>MNAIGNFLVGTPVFTIFICLALGYLLGKLKIGSFTLGATVGVLIVALLIGQLGVFPRDTLLGDIFFDFFMFAIGYR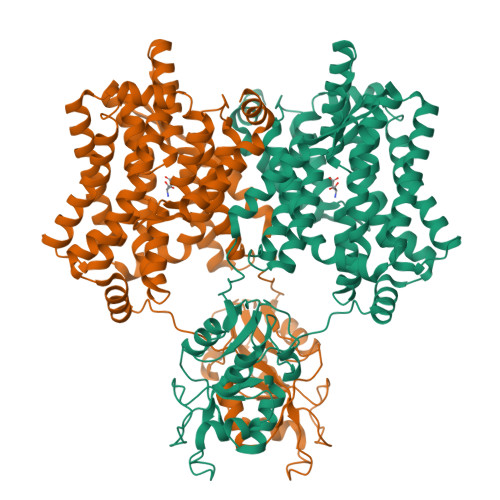VGPSFISSMKKFGAKIVYATLIFLVSAFIVAYACFKMFHIGPGIAAGIIAGGLTQSAVIGSSLETISKLPISDHLKTLYSNQIPIVYTLTYVFGTIGVLIFLRDIMPKLMHIDLKKQAVKTAKELDMIPVPVIVASTHFYTINDGSSLIGQTLGTVNTKFAKGLVAAGLNDSADMASVINAGDVLAISGGIDEIGRAVQEFNLLEVTGKTKAYVSKQVVLKKNFSADVLKNAQDKGVLVATLAGDVMDPAQFSTLKPAESVTLVGQKDAVSEVQSQLGRLRAAENIINYSWFALGIALSAALGIVGTKVSGVPIALGGGTASLIVGLVQSIYRDKHAHMDTIPDSLLEFFQSIGLNLFIATVGLSAAKTFISAIQSMGISVLLIGAVISILPHIITFVICYYLMKMEPISIIGAQTGADTLSAALNDVSERVGSDASPFFAAAVAPAYAIGNIFLTLMGPIFIVLLS[2x]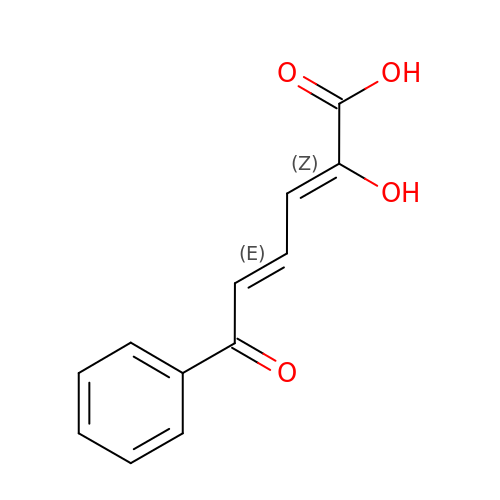(2Z,4E)-2-HYDROXY-6-OXO-6-PHENYLHEXA-2,4-DIENOIC ACID | C12 H10 O4 | RDRDHXDYMGUCKE-KXBBGWRGSA-N> QPRPAFSAIRRNPPMGGNVVIFDTVITN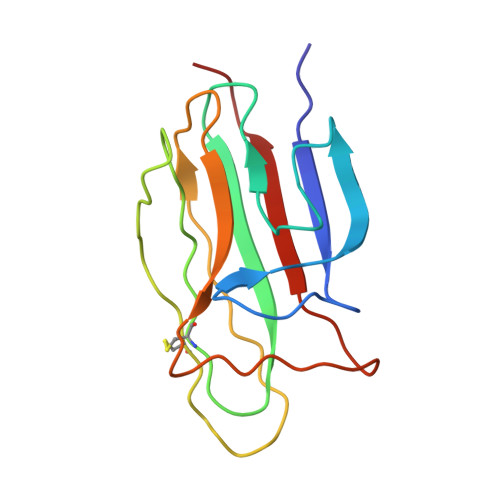QEEPYQNHSGRFVCTVPGYYYFTFQVLSQWEICLSIVSSSRGQVRRSLGFCDTTNKGLFQVVSGGMVLQLQQGDQVWVEKDPKKGHIYQGSEADSVFSGFLIFPSA>[6x]MGHHHHHHGGHMSLSAYKTVVVGTDGSDSSMRAVDRAAQIAGADAKLIIASAYLPQHEDARAADILKDESYKVTGT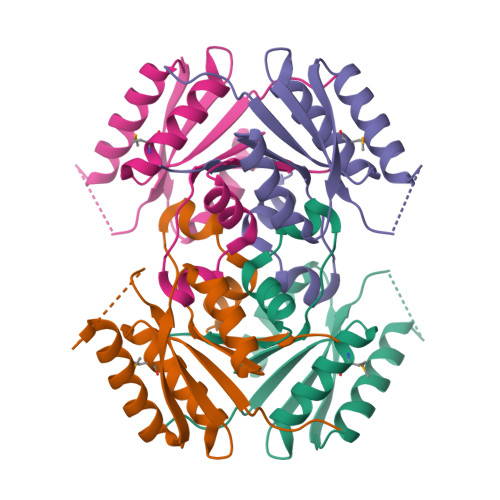APIYEILHDAKERAHNAGAKNVEERPIVGAPVDALVNLADEEKADLLVVGNVGLSTIAGRLLGSVPANVSRRAKVDVLIVHTTEGGS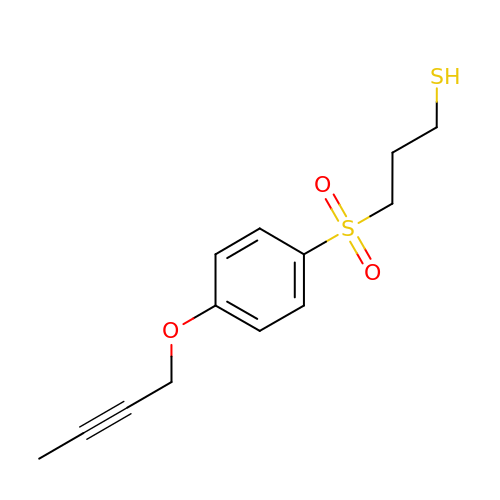3-{[4-(but-2-yn-1-yloxy)phenyl]sulfonyl}propane-1-thiol | C13 H16 O3 S2 | CARKQNSZFCLNKM-UHFFFAOYSA-N>SNANDKVVQKDDSKAETGIMTKNQISSNYYKTVLPYKASKSRGLVVSNIYSRYDINELES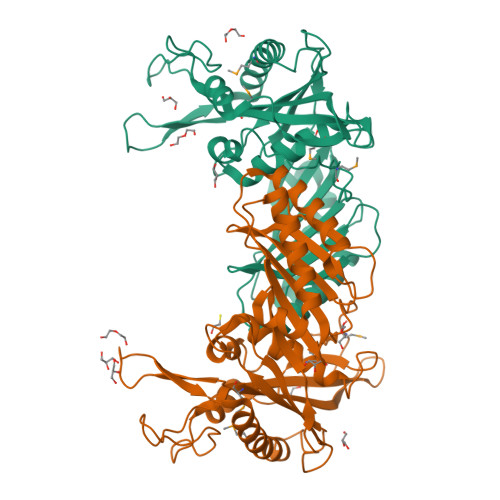GLMRVSQNKYSPDNYLFQEGQYLDKETLEKWLDRKSDKNPNGLNPASNGNGENRKPIYLAHILEQDYLKQTDKDTVALGGISIALAMNSVDYYQKEKYGDTYEQPISDSELLAQGKEMSATVLNRIRQTKGLENVPVTIAIYKQGARDAVAPGNYIAYATANGDSLSNWKDIDEKNYVLPSTESAKDHKTDNDNFLNFKKAIEDYYPNFTGVVGRGRYEDGQLAELNIDIPLQFYGEAEIIGFTQYVTDLVGQHIPKTADLQVNISTSDGPAALITRKANEDAATAHIYD[4x]(3S,4R)-1-[1-(2-chloro-6-cyclopropylbenzene-1-carbonyl)-4-fluoro-1H-indazol-3-yl]-3-hydroxypiperidine-4-carboxylic 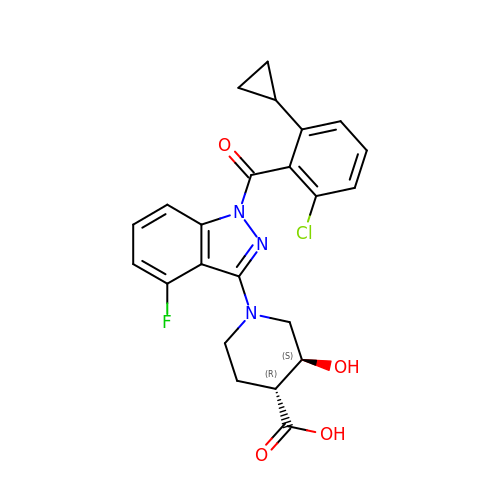acid | C23 H21 Cl F N3 O4 | IBIKHMZPHNKTHM-RDTXWAMCSA-N4-(2-AMINOPHENYL)-4-OXOBUTANOIC 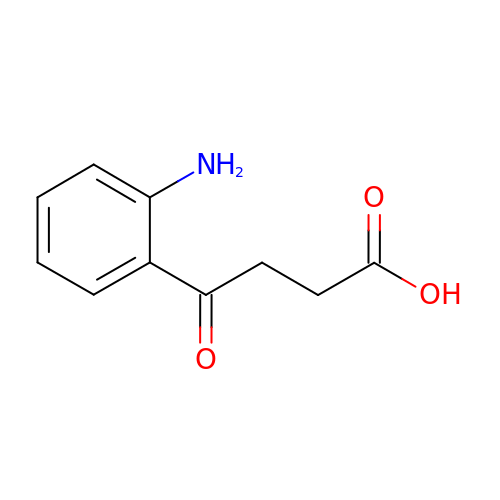ACID | C10 H11 N O3 | BIASMBPERGWEBX-UHFFFAOYSA-N>APHPRVQSPEYVNWTTFKANGVNLGGWLVQESTIDSQFWGTYSGGADDEWGLCEHLGSRCGPVLEHRYATYITERDIDKLASVGVGVLRIPTTYAAWIKLPGSQLYSGNQTAYLKQIADYAITKYGMHIIVDVHSLPGGTNGLTIGEASGHWGWYYNETAFDYSMQVIDAVISFVQNSGSPQSYTIEPMNEPTDNPDMSVFGTPAALSDRGATWVLKYIRAVIDRVASVNPNIPVMFQGSFKPEQYWSNQLPADANLVFDV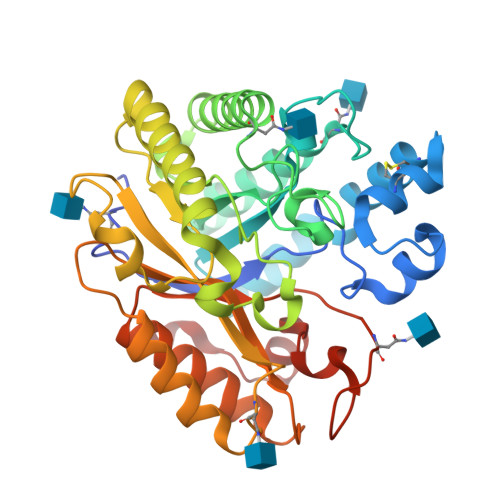HTYYFERNVTSETLPARLYADAQSKAGDGKFPVFTGEWAIQTLYQNSFALRERNVNAGLDAMYKYSQGSCYWTAKFSGNATVNGQGTQADYWNFEYFIDHGYIDLTRFHDTK[2x]> MASMTGGQQMGRGSMSRDPLPFFPPLYLGGPEITTENCEREPIHIPGSIQPHGALLTADGHSGEVLQMSLNAATFLGQEPTVLRGQTLAALLPEQWPALQAALPPGCPDALQYRATLDWPAAGHLSLTVHRVGELLILEFEPTEAWDSTGPHALRNAMFALESAPNLRALAEVATQTVRELTGFDRVMLYKFAPDATGEVIAEARREGLHAFLGHRFPASDIPAQARALYTRHLLRLTADTRAAAVPLDPVLNPQTNAPTPLGGAVLRATSPMAMQYLRNMGVGSSLSVSVVVGGQLW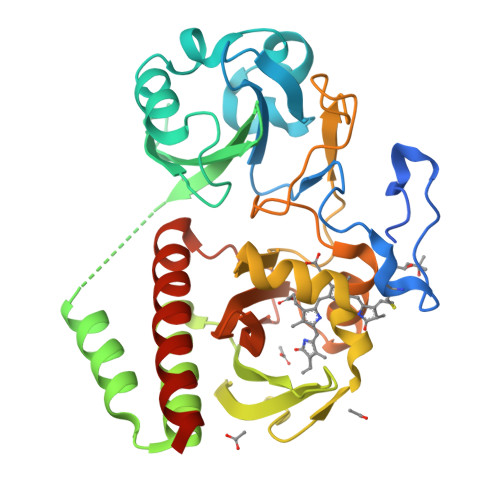GLIACHHQTPYVLPPDLRTTLEYLGRLLSLQVQVKEALEHHHHHH> GTSTQTKAGSLTIVGTGIESIGQMTLQALSYIEAAAKVFYCVIDPATEAFILTKNKNCVDLYQYYDNGKSRLNTYTQMSELMVREVRKGLDVVGVFYGHPGVFVNPSHRALAIAKSEGYRARMLPGVSAEDCLFADLCIDPSNPGCLTYEASDFLIRDRPVSIHSHLVLFQVGCVGIADFNFTGFDNNKFGVLVDRLEQEYGAEHPVVHYIAAMMPHQDPVTDKYTVAQLREPEIAK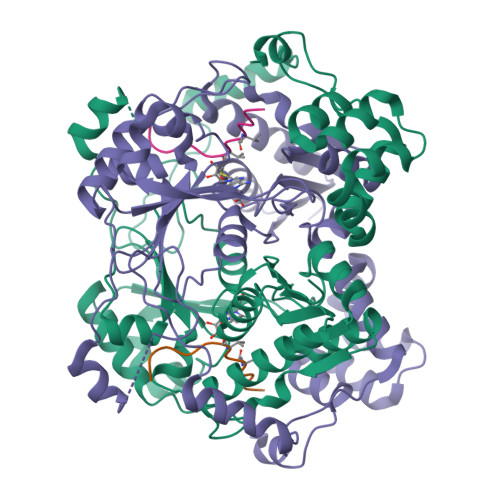RVGGVSTFYIPPKARKASNLDIIRRLELLPAGQVPDKKARIYPANQWEPDVPEVEPYRPSDQAAIAQLADHAPPEQYQPLATSKAMSDVMTKLALDPKALADYKADHRAFAQSVPDLTPQERAALELGDSWAIRCAMKNMPSSLLDAARESGEEASQNGFPWVIVVGVPGVIGSVMSTE;> GFPWVIVVGVPG4-(2-azanylethyl)benzenesulfonic acid | C8 H11 N O3 S | 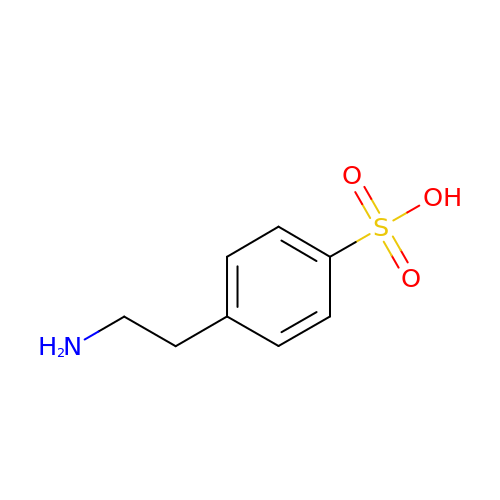RYBFWJVHZIKGQJ-UHFFFAOYSA-N> GSKKKIDILLKAVGDTPIMKTKKWAVERTRTIQGLIDFIKKFLKLVASEQLFIYVNQSFAPSPDQEVGTLYECFGSDGKLVLHYCKSQAWG;> MTDDKD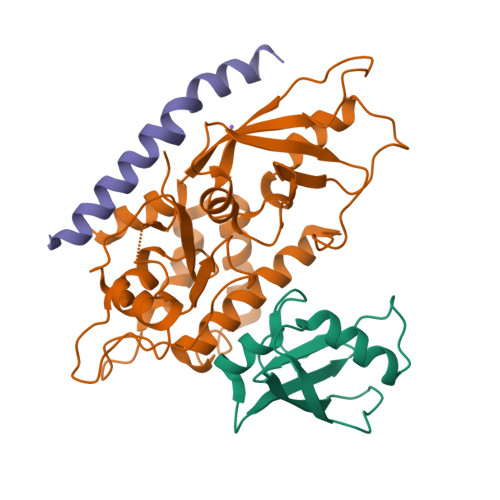VLRDVWFGRIPTCFTLYQDEITEREAEPYYLLLPRVSYLTLVTDKVKKHFQKVMRQEDISEIWFEYEGTPLKWHYPIGLLFDLLASSSALPWNITVHFKSFPEKDLLHCPSKDAIEAHFMSCMKEADALKHKSQVINEMQKKDHKQLWMGLQNDRFDQFWAINRKLMEYPAEENGFRYIPFRIYQTTTERPFIQKLFRPVAADGQLHTLGDLLKEVCPSAIDPEDGEKKNQVMIHGIEPMLETPLQWLSEHLSYPDNFLHISIIPQPTD;> SHMPRWKRHISEQLRRRDRLQRQAFEEIILQYNKLL>GIDPFTSTQQHTEPAEEETLHNIITDTENVQGSFSKHEFQAETKKLLDIVARSLYSEKEVFIRELISNGSDALEKLRHRMITAGGDTAPMEIHLQTDSVKGTFTIQDTGVGMNKEDLVSNLGTIARSGSKAFLDALQNQAEASSSIIGQFGVGFYSAFMVADKVEVYSQSAEADAPGYKWSSDGSGVFEVAEASGVRQGTKIVLHLKDDCKEFSSEDRVKEVVTKYSNFVSFPIFLNGRRLNTLQALWMMEPKDISEWQHEEFYRYVAQAYDKPRYTLHYRADAPLNIRSIFYVPEMKPSMFDVSREMGSSVALYSRKILIQTKATDILPKWLRFLRGVVDSEDIPLNLSRELLQESALIRKLRDVLQQRVIRFLLDQSKKDPEKYARFFEDYGLFMREGIVTTGEQSVKEDIAKLLRFESSALPAGQQTSLMEYSSRMKAGTRNIYYLCAPNRHLAEHSPYFEAMKQKDMEVLFCFEQFDELTLLHLREFDRKKLISAETDIVVDHYKEEKFQDSKPASERLSSEQAEDLLAW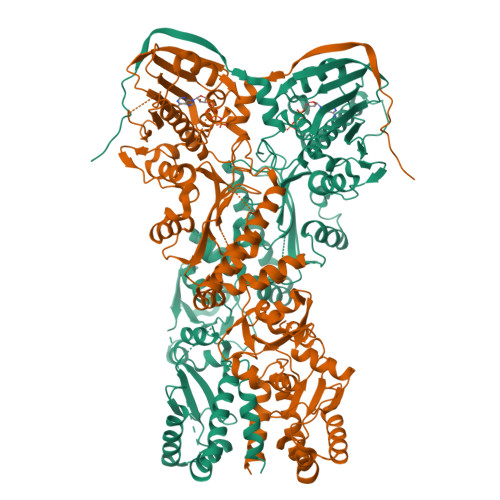MRNALVQRVTNIKVTPRLDTHPAMITVLEMGAARHFLRTQQLARSSEERAQILQPTLEINTGHDLIKKLHALKDSNPELAQLLLEQIYDNAMIAAGLNEDPRPMISRLNQLLTRALEKH[2x]> KDVKVKVTADGRNINDVI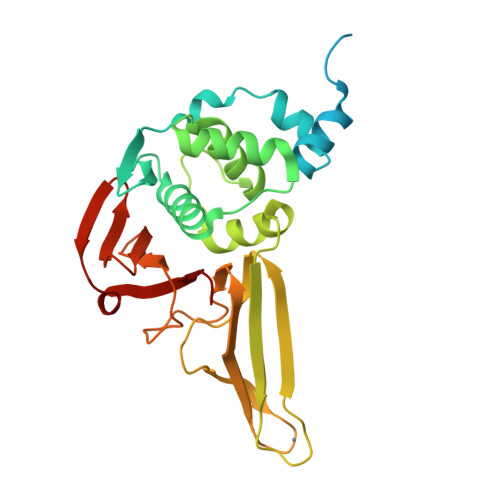VTTAETFDAQLGPSANGAESLVGVVPTPTDGGKVVNTVPDVNWSKHFGFSDAAAFAVLDHSKFAFDSEVVDGKRALADSDNNCWVNATCLALQFLKPTFKYVGWEDLWNKFVTGDVAGFVHLLYYIEGVDKGAKGDVESTLSKLDKYIVSSGSVTVERSTLCDRCNSTVKTVTGAIAEASVILNGHTDGHCPHNFEWRVQVIGVKGDIILLHSGSLLNGPYVYGDAYVAFSGNTDNGHYTVFDNKLSKMYDGIKCVKTTLDTLVASSVVIRNGSY[6-chloranyl-4-[(5-methyl-1H-pyrazol-3-yl)amino]quinazolin-2-yl]-[(3R)-3-methylpiperazin-1-yl]methanone 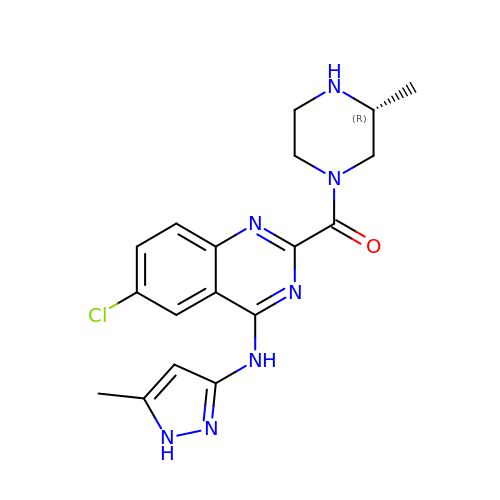| C18 H20 Cl N7 O | WQTMYTFWTYPJST-LLVKDONJSA-N> MPCSEETPAISPSKRARPAEVGGMQLRFARLSEHATAPTRGSARAAGYDLYSAYDYTIPPMEKAVVKTDIQIALPSGCYGRVAPRSGLAAKHFIDVGAGVIDEDYRGNVGVVLFNFGKEKFEVKKGDRIAQLICE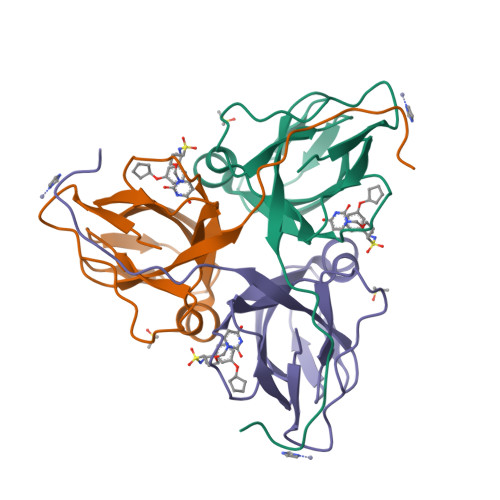RIFYPEIEEVQALDDTERGSGGFGSTGKN3-DEOXY-D-ARABINO-HEXONIC 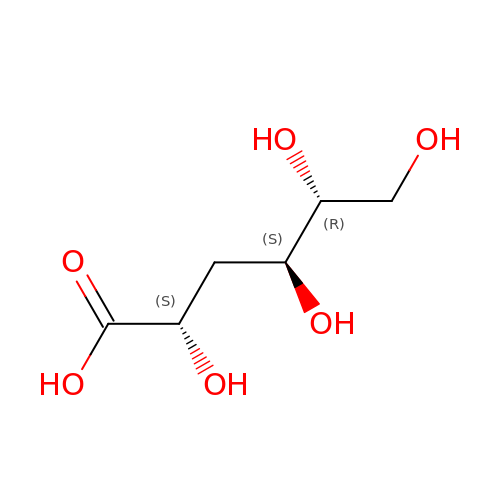ACID | C6 H12 O6 | YGMNHEPVTNXLLS-VAYJURFESA-N> VPATRILLLVLAVIIYGTAGFHFIEGESWTVSLYWTFVTIAAVGYGDYSPHTPLGMYFTCTLI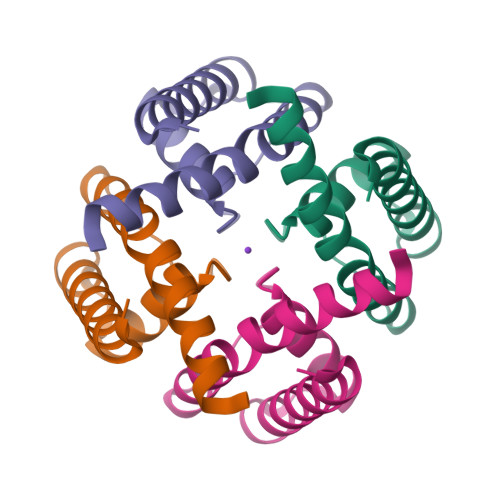VLGIGTFAVAVERLLEFLI>MNGAIKVGA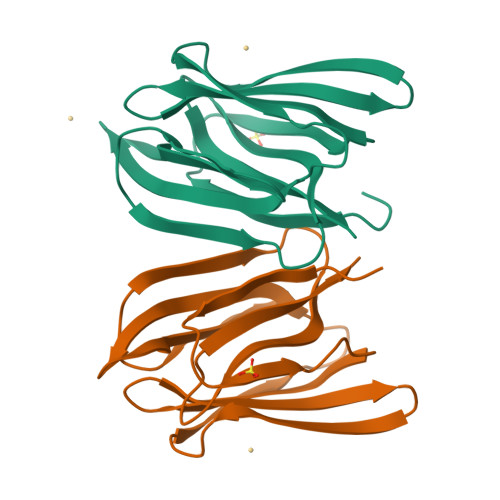WGGNGGSAFDMGPAYRIISVKIFSGDVVDGVDVTFTYYGKTETRHYGGSGGTPHEIVLQEGEYLVGMAGEVANYHGAVVLGKLGFSTNKKAYGPFGNTGGTPFSLPIAAGKISGFFGRGGKFLDAIGVYLEP[2x]> GPGSAVAVDPAPV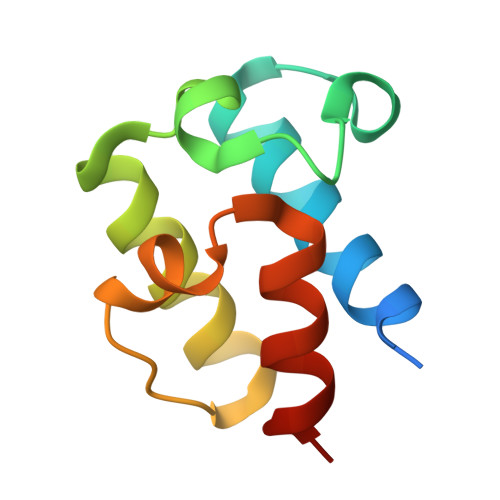ARALREELARTLYCEPGDIDDEASFNTLGLDSILGVEFVAFVNQTYGLDEKAGILYDHPSLAALSRHVAGRAAPV>MNTPEHMTAVVQRYVAALNAGDLDGIVALFADDATVYETSQDRTYTGTAAIREFYANSLKLPLAVELTQEVRANRNEAAFAFTVSFEYQGRKTVVAPIDHFRFNGAGKVVSMRALFGEKNIHAGAGS[4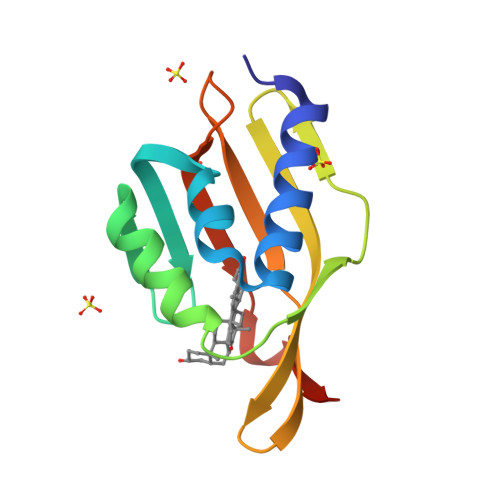x]> MAQRGIREYDAKNLLARYLPEYLDDFSYKGNLALVGPETDIEGLEAENPWLKTTRLVVKPDQLFGKRGKLGLVLLDADWEEAKEYLNEKMGLEVTIGGITGRLSYFLIEPFTPHKEEYYVAISSDYEGDNIFFSMDGGVGVEENWEKVISIHVDSLEGIDALDVGSKLPAELGDKRALVEEFITALWRFYSDTGFAYVEINPFTFSGRGIVPLDMVAKLDDAEEYWQKKRWSELAFPEPFGRTPSKEELFIKEIDSKTGASLKLTILNPEGRVWTMVAGGGASVIYADTICDLGHADEMANYGEYSGDPNTEETYHYTCTILDLMTRSKNPNGKVLLIGGAIANFTDVAKTFKGVVMALEEYQQKLQEADIEIYVRRGGPNYEQGLKLMRDLGKRLGVPIQV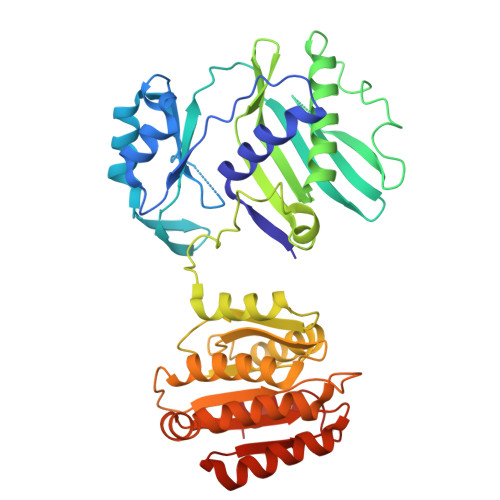HGPETHMTRIVPLALEENQ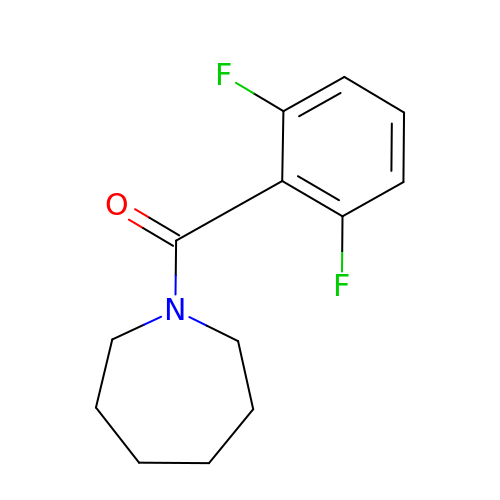(azepan-1-yl)(2,6-difluorophenyl)methanone | C13 H15 F2 N O | RRINWFXOXXUQGK-UHFFFAOYSA-N> GAGVSISAQNLIKNEKFATEVTNKVTNPSKATAGEWFIMNNEADGVTTIAWEQTGDAKYPNAMKIDNSGAEKNTSWYKAFLGQRITDGLEKGIYVLTFYAKAKEAGTPVSVYIKQTNEEKNDNGKLNTTFFMRRDYDADAQPNASGAQYNFKIKDADKWTKVVV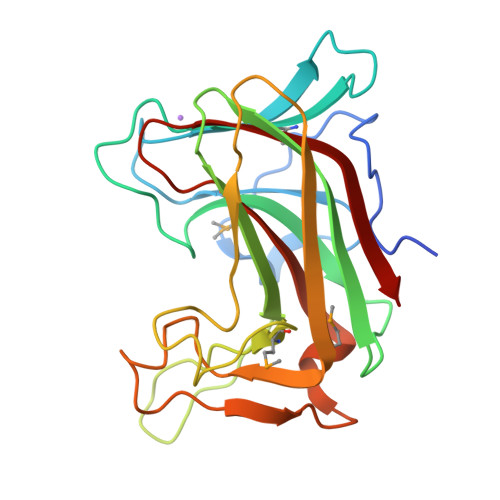YYDMGQVVNAISSKKSNPALEVSDTDDDAAILKDCYVAILGQNKGGVVEISDVTLKKK>[2x]RLVQLSRHSIAFPSPEGALREPNGLLALGGDLSPARLLMAYQRGIFPWFSPGDPI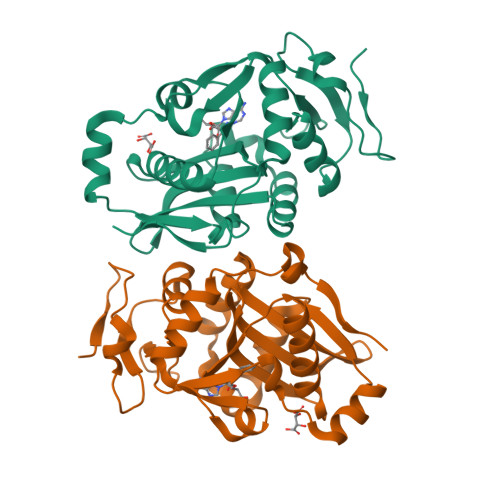LWWSPDPRAVLWPESLHISRSMKRFHKRSPYRVTMNYAFGQVIEGCASDREEGTWITRGVVEAYHRLHELGHAHSIEVWREDELVGGMYGVAQGTLFCGESMFSRMENASKTALLVFCEEFIGHGGKLIDCQVLNDHTASLGACEIPRRDYLNYLNQMRLGRLPNNFWVPRCLFSPQE> PCTLEYMRCKQDS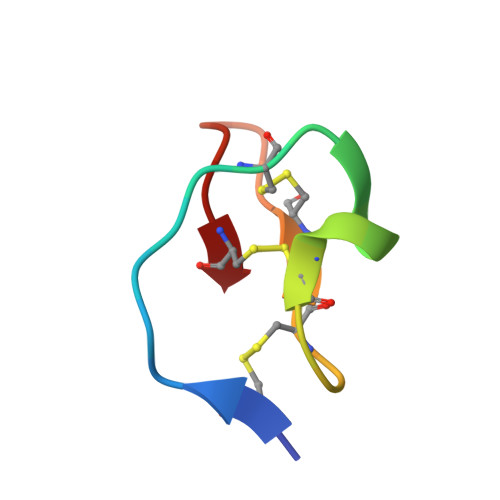DCLAGCVCGPNGFCG>MGSSHHHHHHSSGENLYFQGHMSSTFEPATDSPLPVPGVQYFLQHVQSGKYVHPHGGSDMPGNDTALVLHHGFDEKRDALRWVFVNDAENKHQLKHYSSGKFVHPKGGKVGKEATLVVHSSPGRPETMIEMVQEDGRTYLRHTDSDYYVHPHGGSPNPGDNTRLVYYSGYRPSLAFLAIPAETLFVDRIEIHQAQALESINTITSLSDEHRNDTDQPVQTSISVALEESLQDSAQLSFERCFGLKVGSEFEVGLPLVGKTKVSVQFSGSWKSSTIKGEVRTSAVKVQINEHVTIPPGK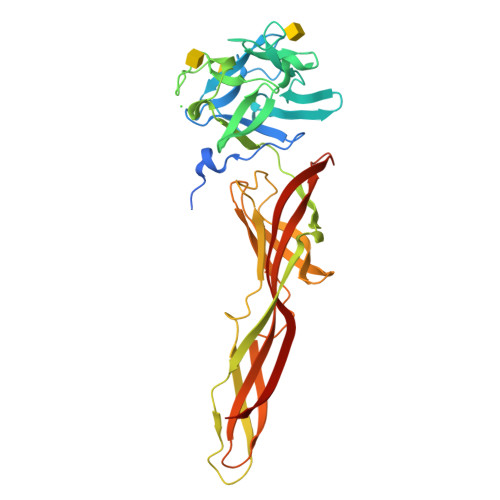CVQIRIDTRRCTKTAPATMYLRTASGIEVQRETTVTSTYHYDQEVHVVPVTN[2x]>STLRLLISD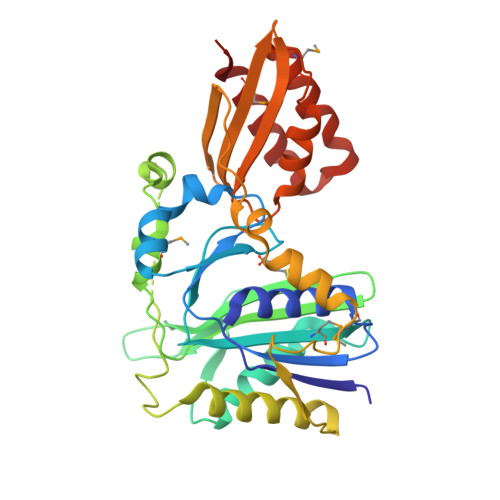SYDPWFNLAVEECIFRQMPATQRVLFLWRNADTVVIGRAQNPWKECNTRRMEEDNVRLARRSSGGGAVFHDLGNTCFTFMAGKPEYDKTISTSIVLNALNALGVSAEASGRNDLVVKTVEGDRKVSGSAYRETKDRGFHHGTLLLNADLSRLANYLNPDKKKLAAKGITSVRSRVTNLTELLPGITHEQVCEAITEAFFAHYGERVEAEIISPNKTPDLPNFAETFARQSSWEWNFGQAPAFSHLLDERFTWGGVELHFDVEKGHITRAQVFTDSLNPAPLEALAGRLQGCLYRADMLQQECEALLVDFPEQEKELRELSAWMAGAVR[3x]> EDPFGPGCEEAGCPEG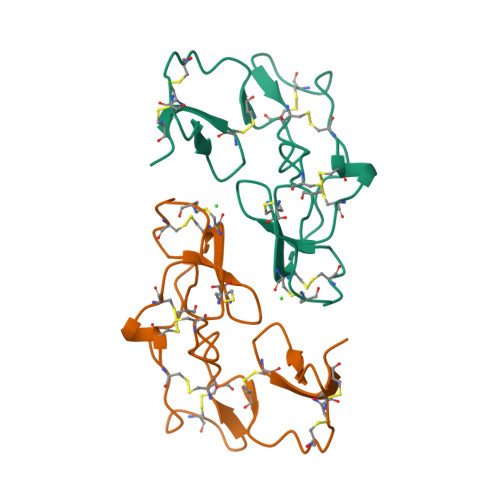SACNIITDRCTCSGVRCRVHCPHGFQRSRYGCEFCKCRLEPMKATCDISECPEGMMCSRLTNKCDCKIDINCRKTCPNGLKRDKLGCEYCECRPKRKLIPRLS>[4x]MAHHHHHHMSQLANVIRFLSADAVQKANSGHPGAPMGMAEMAETLWTKFLNHNPANPKFYNRDRFVLSNGHASMLLYSLLHLTGYNLSIEDLKNFRQLHSKTPGHPEYGYTDGVETTTGPLGQGIANAVGMALAEKILAAEFNKDGLNIVDHYTYVFMGDGCLMEGVSHEACSLAGTLGLGKLIVLYDDNNISIDGKVDGWFTENIPQRFESYGWHVVPNVNGHDTAAIQTAIEA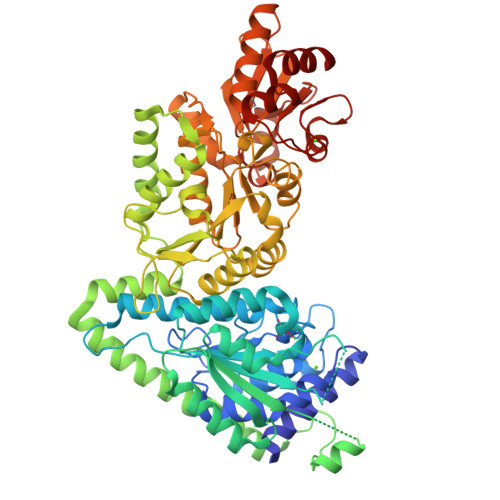ARAETGKPSIICCKTLIGKGSANKEGSHKTHGAPLGADEIEATRKHLGWAYPAFEIPQEIYDAWNAKEKGAKLEAGWNELFAQYQAKYPAEAAEFVRRMDKKLPENFDEYVQTALKEVCAKAETVATRKASQNSIEILAKELPELVGGSADLTPSNLTDWSNSVSVTRDKGGNYIHYGVREFGMGAIMNGLVLHGGVKPFGATFLMFSEYERNALRMAALMKINPVFVFTHDSIGLGEDGPTHQPIEQTATLRLIPNMDVWRPCDTAESLVAWAEAAKAEDHPSCLIFSRQNLKFQARSEQQLNDIKRGAYVISEAQGNAQAVIIATGSEVGLAVEAQKVLAGQGIAVRVVSMPSTSVFDRQDAAYQAAVLPEGLPRIAVEAGHTNGWYKYVGLNGAVVGINRFGESAPADLLFKAFGFTVDNVVDTVKSVL>[2x]MRLTDTNLLEVLNSEEYSGVLKEFREQRYSKKAILYTPNTERNLVFLVKSGRVRVYLAYEDKEFTLAILEAGDIFCTHTRAFIQAMEDTTILYTDIRNFQNIVVEFPAFSLNMVKVLGD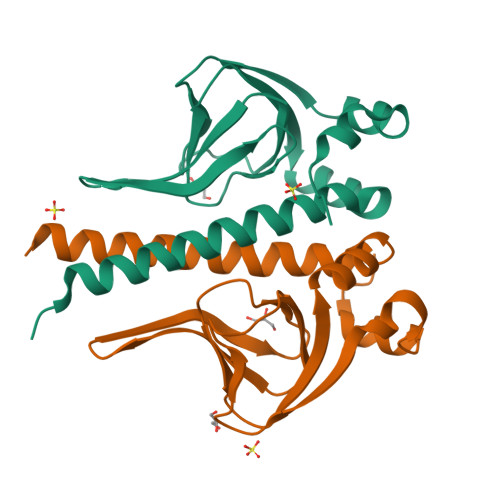LLKNSLTIINGLVFLEHHHHHH> MNLMTTITGVVLAGGKARRMGGVDKGLLELNG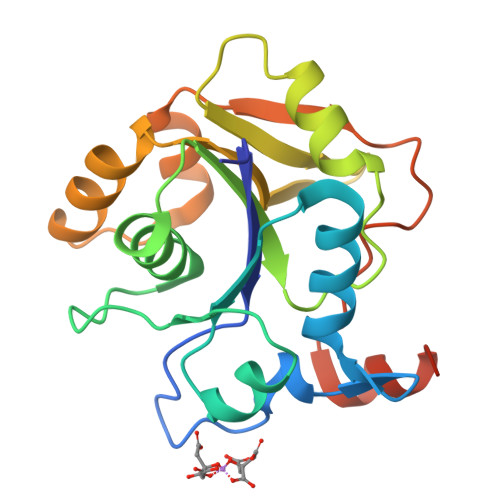KPLWQHVADALMTQLSHVVVNANRHQEIYQASGLKVIEDSLADYPGPLAGMLSVMQQEAGEWFLFCPCDTPYIPPDLAARLNHQRKDAPVVWVHDGERDHPTIALVNRAIEPLLLEYLQAGERRVMVFMRLAGGHAVDFSDHKDAFVNVNTPEELARWQEKRSHHHHHH> MGSDYKDHDGDYKDHDIDYKDDDDKGSGSLEVLFQGPMDPLNESTVNVYLPDSYLKGVISFSETNAIGSCLLKRPYLKNDNTAKVAIENPVIEHVRLKNAVNSKMKISDYKVVEPVNMQHEIMKNVHSCELTLLKQFLTRSKNISTLKLNMICDWLQLKSTSDDTSILSFIDVEFIPSWVSNWFSNWYNLNKLILEFRREEVIRTGSILCRSLGKLVFIVSSYGCIVKSNKSKRVSFFTYNQLLTWKDVMLSRFNANFCIWVSNSLNENQEGLGLRSNLQGMLTNKLYETVDYMLSLCCNEGFSLVKEFEGFIMSEILRITEHAQFSTRFRNTLLNGLTDQLTKLKNKNRLRVHSTVLENNDYPMYEVVLKLLGDTLRCIKLLINKNLENAAELYYIFRIFGHPMVDERDAMDAVKLNNEITKILRLESLTELRGAFILRIIKGFVDNNKRWPKIKNLKVLSKRWTMYFKAKNYPSQLELSEQDFLELAAIQFEQEFSVPEKTNLEMVLNDKAISPPKRLIWSVYPKNYLPETIKNRYLEETFNASDSLKTRRVLEYYLKDNKFDQKELKSYVVRQEYLNDKEHIVSLTGKERELSVGRMFAMQPGKQRQ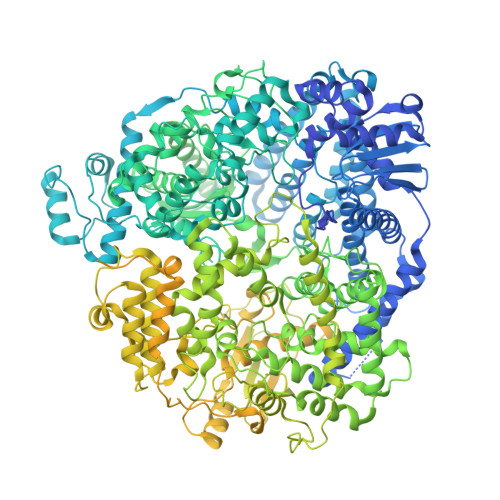IQILAEKLLADNIVPFFPETLTKYGDLDLQRIMEIKSELSSIKTRRNDSYNNYIARASIVTDLSKFNQAFRYETTAICADVADELHGTQSLFCWLHLIVPMTTMICAYRHAPPETKGEYDIDKIEEQSGLYRYHMGGIEGWCQKLWTMEAISLLDVVSVKTRCQMTSLLNGDNQSIDVSKPVKLSEGLDEVKADYRLAVKMLKEIRDAYRNIGHKLKEGETYISRDLQFISKVIQSEGVMHPTPIKKVLRVGPWINTILDDIKTSAESIGSLCQELEFRGESIIVSLILRNFWLYNLYMHESKQHPLAGKQLFKQLNKTLTSVQRFFEIKRENEVVDLWMNIPMQFGGGDPVVFYRSFYRRTPDFLTEAISHVDILLKISANIKNETKVSFFKALLSIEKNERATLTTLMRDPQAVGSERQAKVTSDINRTAVTSILSLSPNQLFSDSAIHYSRNEEEVGIIAENITPVYPHGLRVLYESLPFHKAEKVVNMISGTKSITNLLQRTSAINGEDIDRAVSMMLENLGLLSRILSVVVDSIEIPIKSNGRLICCQISRTLRETSWNNMEIVGVTSPSITTCMDVIYATSSHLKGIIIEKFSTDRTTRGQRGPKSPWVGSSTQEKKLVPVYNRQILSKQQREQLEAIGKMRWVYKGTPGLRRLLNKICLGSLGISYKCVKPLLPRFMSVNFLHRLSVSSRPMEFPASVPAYRTTNYHFDTSPINQALSERFGNEDINLVFQNAISCGISIMSVVEQLTGRSPKQLVLIPQLEEIDIMPPPVFQGKFNYKLVDKITSDQHIFSPDKIDMLTLGKMLMPTIKGQKTDQFLNKRENYFHGNNLIESLSAALACHWCGILTEQCIENNIFKKDWGDGFISDHAFMDFKIFLCVFKTKLLCSWGSQGKNIKDEDIVDESIDKLLRIDNTFWRMFSKVMFEPKVKKRIMLYDVKFLSLVGYIGFKNWFIEQLRSAELHEIPWIVNAEGDLVEIKSIKIYLQLIEQSLFLRITVLNYTDMAHALTRLIRKKLMCDNALLTPISSPMVNLTQVIDPTTQLDYFPKITFERLKNYDTSSNYAKGKLTRNYMILLPWQHVNRYNFVFSSTGCKVSLKTCIGKLMKDLNPKVLYFIGEGAGNWMARTACEYPDIKFVYRSLKDDLDHHYPLEYQRVIGELSRIIDSGEGLSMETTDATQKTHWDLIHRVSKDALLITLCDAEFKDRDDFFKMVILWRKHVLSCRICTTYGTDLYLFAKYHAKDCNVKLPFFVRSVATFIMQGSKLSGSECYILLTLGHHNSLPCHGEIQNSKMKIAVCNDFYAAKKLDNKSIEANCKSLLSGLRIPINKKELDRQRRLLTLQSNHSSVATVGGSKIIESKWLTNKASTIIDWLEHILNSPKGELNYDFFEALENTYPNMIKLIDNLGNAEIKKLIKVTGYMLVSKK3-[5-(3-cyclohexyl-3,5,8,10-tetrazatricyclo[7.3.0.0^{2,6}]dodeca-1(9),2(6),4,7,11-pentaen-4-yl)furan-2-yl]propanenitrile | C21 H21 N5 O | 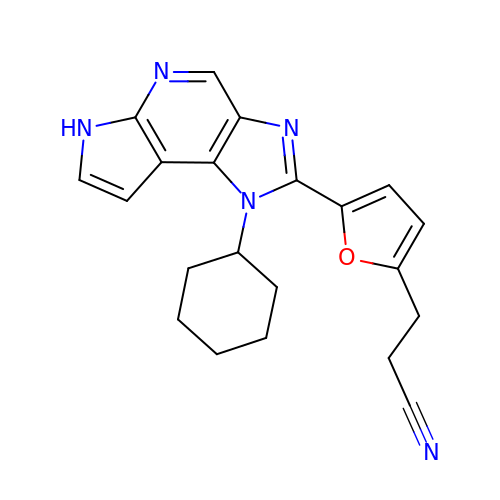PLKGAHIHTTYWEV-UHFFFAOYSA-N> MLRWITAGESHGRALVAVVEGMVAGVHVTSADIADQLARRRLGYGRGARMTFERDAVTVLSGIRHGSTLGGPIAIEIGNTEWPKWETVMAADPVDPAELADVARNAPLTRPRPGHADYAGMLKYGFDDARPVLERASARETAARVAAGTVARAFLRQALGVEVLSHVISIGASAPYEGPPPRAEDLPAIDASPVRAYDKAAEADMIAQIEAAKKDGDTLGGVVEAVALGLPVGLGSFTSGDHRLDSQLAAAVMGIQAIKGVEIGDGFQTARRRGSRAHDEMYPGPDGVVRSTNRAGGLEGGMTNGQPLRVRAAMKPISTVPRALATVDLATGDEAVAIHQRSDVC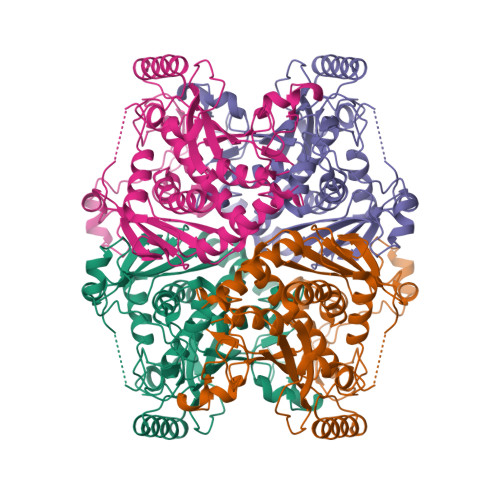AVPAAGVVVETMVALVLARAALEKFGGDSLAETQRNIAAYQRSVADREAPAARVSG> MGVQFGDFIPKNIISFEDLKGKKVAIDGMNALYQFLTSIRLRDGSPLRNRKGEITSAYNGVFYKTIHLLENDITPIWVFDGEPPKLKEKTRKVRREMKEKAELKMKEAIKKEDFEEAAKYAKRVSYLTPKMVENCKYLLSLMGIPYVEAPSEGEAQASYMAKKGDVWAVVSQDYDALLYGAPRVVRNLTTTKEMPELIELNEVLEDLRISLDDLIDIAIFMGTDYNPGGVKGIGFKRAYELVRSGVAKDVLKKEVEYYDEIKRIFKEPKVTDNYSLSLKLPDKEGIIKFLVDENDFNYDRVKK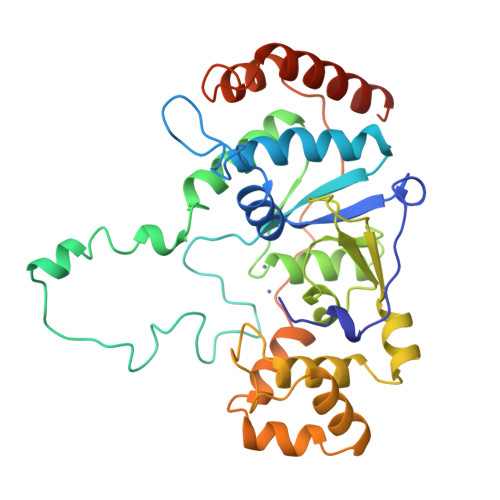HVDKLYNLIANKTKQKTLDAWFK>MTGMSREEVESLIQEVLEVYPEKARKDRNKHLAVNDPAVTQSKKCIISNKKSQPGLMTIRGCAYAGSKGVVWGPIKDMIHISHGPVGCGQYSRAGRRNYYIGTTGVNAFVTMNFTSDFQEKDIVFGGDKKLAKLIDEVETLFPLNKGISVQSECPIGLIGDDIESVSKVKGAELSKTIVPVRCEGFRGVSQSLGHHIANDAVRDWVLGKRDEDTTFASTPYDVAIIGDYNIGGDAWSSRILLEEMGLRCVAQWSGDGSISEIELTPKVKLNLVHCYRSMNYISRHMEEKYGIPWMEYNFFGPTKTIESLRAIAAKFDESIQKKCEEVIAKYKPEWEAVVAKYRPRLEGKRVMLYIGGLRPRHVIGAYEDLGMEVVGTGYEFAHNDDYDRTMKEMGDSTLLYDDVTGYEFEEFVKRIKPDLIGSGIKEKFIFQKMGIPFREMHSWDYSGPYHGFDGFAIFARDMDMTLNNPCWKKLQAPWEASEGAEKVAASA[2x];>[2x]MSQQVDKIKASYPLFLDQDYKDMLAKKRDGFEEKYPQDKIDEVFQWTTTKEYQELNFQREALTVNPAKACQPLGAVLCALGFEKTMPYVHGSQGCVAYYRSYFNRHFREPVSCVSDSMTEDAAVFGGQQNMKDGLQNCKATYKPDMIAVSTTCMAEVIGDDLNAFINNSKKEGF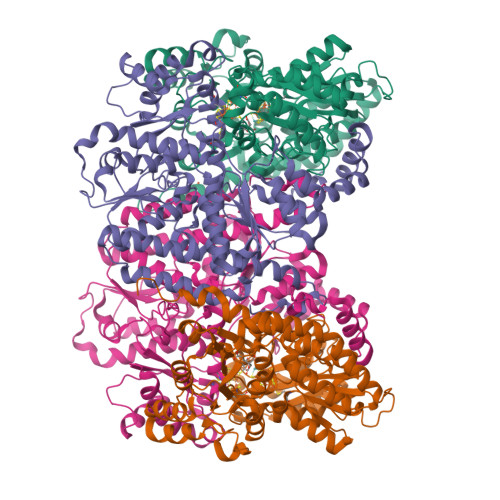IPDEFPVPFAHTPSFVGSHVTGWDNMFEGIARYFTLKSMDDKVVGSNKKINIVPGFETYLGNFRVIKRMLSEMGVGYSLLSDPEEVLDTPADGQFRMYAGGTTQEEMKDAPNALNTVLLQPWHLEKTKKFVEGTWKHEVPKLNIPMGLDWTDEFLMKVSEISGQPIPASLTKERGRLVDMMTDSHTWLHGKRFALWGDPDFVMGLVKFLLELGCEPVHILCHNGNKRWKKAVDAILAASPYGKNATVYIGKDLWHLRSLVFTDKPDFMIGNSYGKFIQRDTLHKGKEFEVPLIRIGFPIFDRHHLHRSTTLGYEGAMQILTTLVNSILERLDEETRGMQATDYNHDLVR> LAGAETEIDEVTPNHVAIIIDGHRKWAKSRGVTVQEGHQTGVNNWKHIISRASQLGIKLLTIWALSPQNFNRSKMEVDFLMRIYEDFLRSDVKELVTSQQDIQFSAIGDKSRLPEYLQDAISYAEGLSQANKGMHFILAVAYGGREDIVEAARKIAAKVEHGILRPDDIDEATFEQHLMTNITKFPSPDLLIRAAGEQRLSNFFLWQLPFTEFYFTPKLFPDFGEADLLDALASYRCRYRGFGERKGIHEASA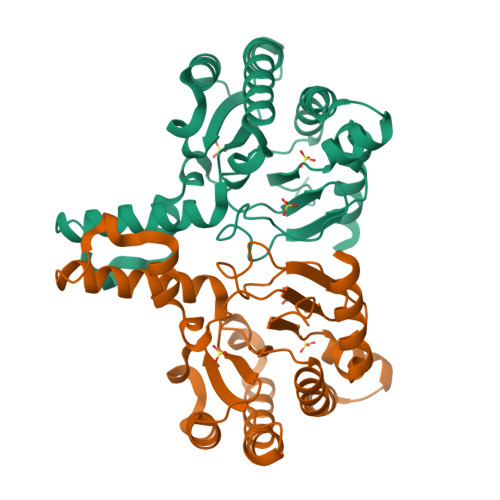WSHPQFEK> AAWVKGGAADVDAAVEAAADLLAASRVPVLAGLSAEVSALRAAYRLAETLGASLDPVSGPSVYAELGALSAGGAMSTTRAETIGRADVILIVGNRPWDGELIAEIAAAAPSRGRAAGAERALLSLGGPQNGAIRHVAYAADAG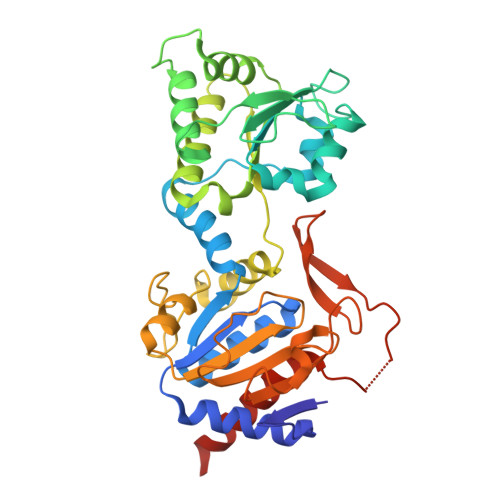GLTISLGHLRAFAKGHLAGEAAFADLAKRLFAAQYGVIVYDPEEVGELGAEMLQGLIRDLNESTRFFALTLADPFQGRAAVQLSAWTTGQAPRVGFGRHQPEHDSWRFDSARQIAAGEADAALWLASLPAPRPAWLGSLPTIAIVGEGSQEAAGETAEVVITVGVPGQSVGGALWNDRRGVIAYAEASDPAKTPAETETAAGVLTRIRDRLIEKGVSC> AMAISDPEETLMDSTTATAELGWMVHPPSGW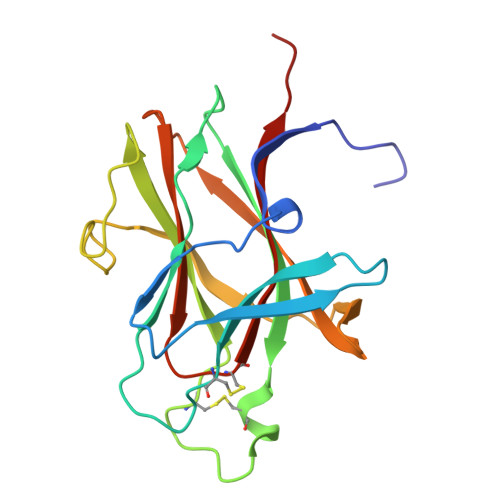EEVSGYDENMNTIRTYQVCNVFESSQNNWLRTKFIRRRGAHRIHVEMKFSVRDCSSIPSVPGSCKETFNLYYYEADFDLATKTFPNWMENPWVKVDTIAADESISQVDLGGRVMKINTEVRSFGPVSRNGFYLAFQDYGGCMSLIAVRVFYRKCPR>[2x]MARIRAVQGDITEFQGDAIVNAANNYLKLGAGVAGAILRKGGPSIQEECDRIGKIRVG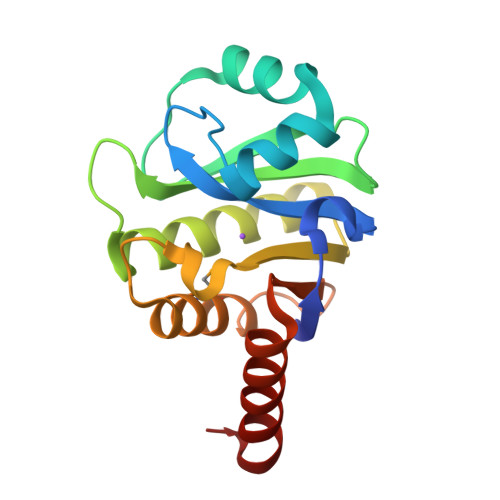EAAVTGAGNLPVRYVIHAAVLGDEPASLETVRKATKSALEKAVELGLKTVAFTALGAWVGGLPAEAVLRVMDEEIKKAPDTLEVTGVHGTEKSAEAHRRALLEHHHHHH5-cyclopropyl-6-(2,6-dimethylpyridin-4-yl)-~{N}-[(3~{R},4~{R})-3-fluoranylpiperidin-4-yl]-1~{H}-indazol-3-amine 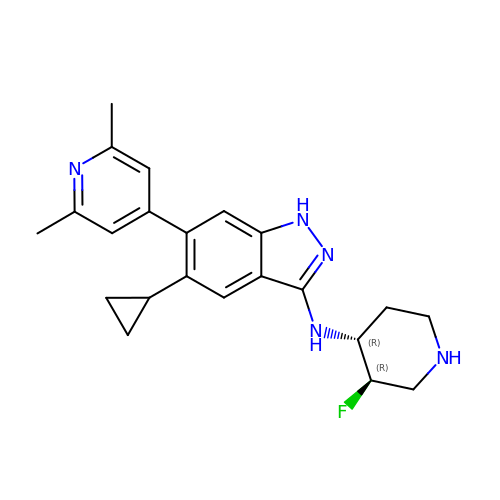| C22 H26 F N5 | JUSJRQVEHUHMRQ-WOJBJXKFSA-N>[4x]GPHMDEHYLDNLCIFCGERSEEFTEEGLDLHYWKHCLMLTRCDHCKQVVEISSLTEHLLTECDKKDGFGKCYRCSEAVFKEELPRHIKHKDCNPAKPEKLANRCPLCHENFSPGEE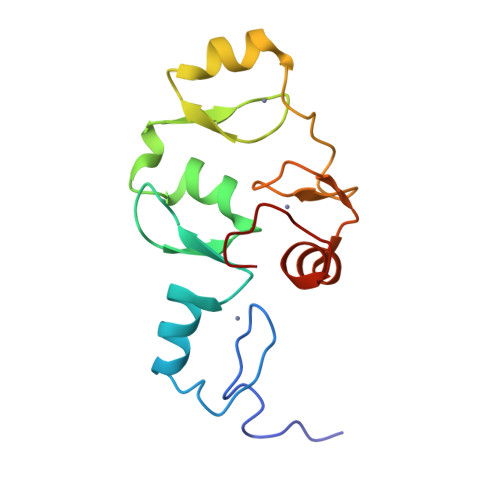AWKAHLMGPAGCTMNLRK>[2x]MGSSHHHHHHSQDPMSLNLVSEQLLAANGLKHQDLFAILGQLAERRLDYGDLYFQSSYHESWVLEDRIIKDGSYNIDQGVGVRAISGEKTGFAYADQISLLALEQSAQAARTIVRDSGDGKVQTLGAVEHSPLYTSVDPLQSMSREEKLDILRRVDKVAREADKRVQEVTASLSGVYELILVAATDGTLAADVRPLV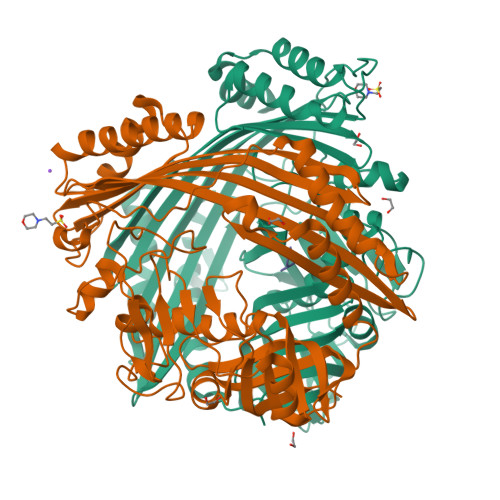RLSVSVLVEEDGKRERGASGGGGRFGYEFFLADLDGEVRADAWAKEAVRMALVNLSAVAAPAGTMPVVLGAGWPGVLLHEAVGHGLEGDFNRRGTSVFSGQVGELVASELCTVVDDGTMVDRRGSVAIDDEGTPGQYNVLIENGILKGYMQDKLNARLMGMTPTGNGRRESYAHLPMPRMTNTYMLPGKSTPQEIIESVEYGIYAPNFGGGQVDITSDKFVFSTSEAYLIENGKVTKPVKGATLIGSGIETMQQISMVGNDLKLDNGVGVCGKEGQSLPVGVGQPTLKVDNLTVGGTA;>[2x]MALAMKVISQVEAQRKILEEAVSTALELASGKSDGAEVAVSKTTGISVSTRYGEVENVEFNSDGALGITVYHQNRKGSASSTDLSPQAIARTVQAALDIARYTSPDPCAGVADKELLAFDAPDLDLFHPAEVSPDEAIELAARAEQAALQADKRITNTEGGSFNSHYGVKVFGNSHGMLQGYCSTRHSLSSCVIAEENGDMERDYAYTIGRAMSDLQTPEWVGADCARRTLSRLSPRKLSTMKAPVIFANEVATGLFGHLVGAIAGGSVYRKSTFLLDSLGKQILPDWLTIEEHPHLLKGLASTPFDSEGVRTERRDIIKDGILTQWLLTSYSARKLGLKSTGHAGGIHNWRIAGQGLSFEQMLKEMGTGLVVTELMGQGVSAITGDYSRGAAGFWVENGEIQYPVSEITIAGNLKDMWRNIVTVGNDIETRSNIQCGSVLLPEMKIAGQ;>[2x]DRVY>GPLGSPGIPGQNTPWSSTELADAFI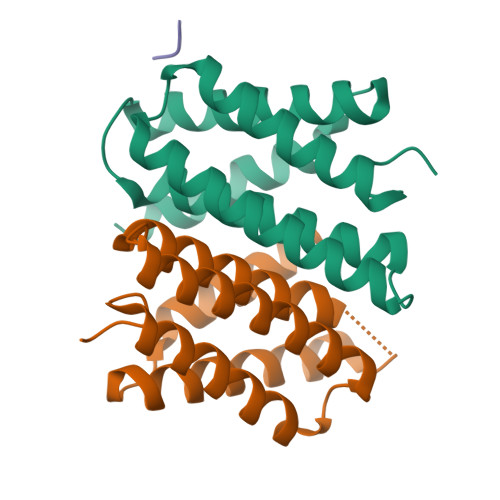NAFMNEAGRTGAFTADQLDDMSTIGDTIKTAMDKMARSNKSSKGKLQALNMAFASSMAEIAAVEQGGLSVDAKTNAIADSLNSAFYQTTGAANPQFVNEIRSLINMFAQSSANEVSYGG[2x];> SYG>[2x]MKNPFSLEGR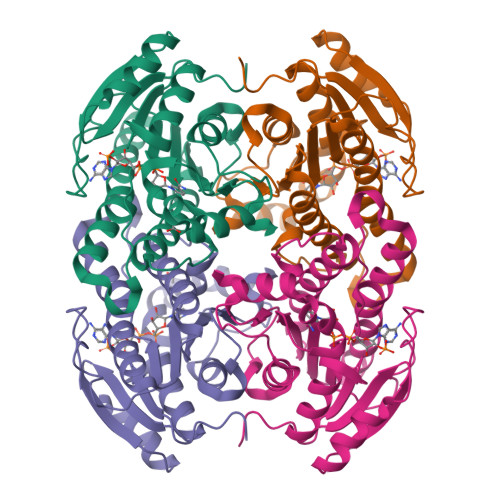KALVTGANTGLGQAIAVGLAAAGAEVVCAARRAPDETLDIIAKDGGNASALLIDFADPLAAKDSFTDAGFDILVNNAGIIRRADSVEFSELDWDEVMDVNLKALFFTTQAFAKELLAKGRSGKVVNIASLLSFQGGIRVPSYTAAKHGVAGLTKLLANEWAAKGINVNAIAPGYIETNNTEALRADAARNKAILERIPAGRWGHSEDIAGAAVFLSSAAADYVHGAILNVDGGWLAR>[2x]MGSDKIHHHHHHMAEFTHLVNERRSASNFLSGHPITKEDLNEMFELVALAPSAFNLQHTKYVTVLDQDV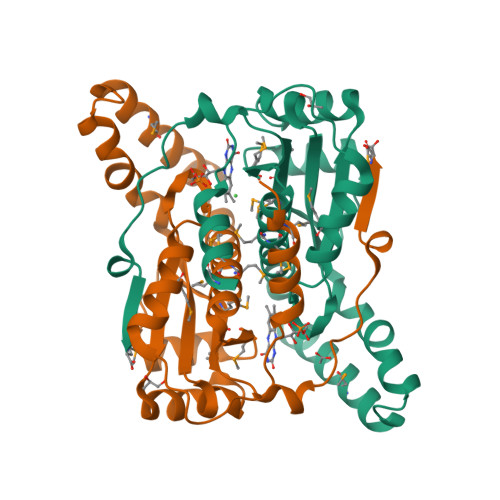KEKLKQAANGQYKVVSSSAVLLVLGDKQAYQQAADIYEGLKVLGILNKQEYDHMVQDTVSFYENRGEQFKRDEAIRNASLSAMMFMLSAAAAGWDTCPMIGFDAEAVKRILNIDDQFEVVMMITIGKEKTESRRPRGYRKPVNEFVEYM>MSDNNQALK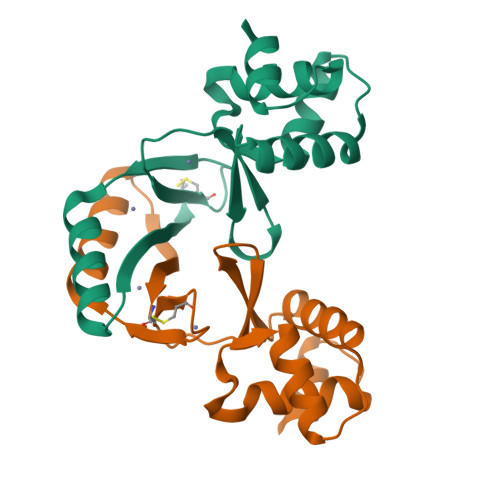DAGLKVTLPRLKILEVLQQPECQHISAEELYKKLIDLGEEIGLATVYRVLNQFDDAGIVTRHHFEGGKSVFELSTQHHHDHLVCLDCGEVIEFSDDVIEQRQKEIAAKYNVQLTNHSLYLYGKCGSDGSCKDNPNAHKPKK[2x]>GMTTLNLNTLSERIKAHKMALVHIVKPPVCTERAQHYTEMYQQHMDKPIPVRRALALAHHLAQRTIWIKHDELIVGNQASEVRAAPIFPEYTVSWIEKEIDDLADRPGAGFAVSEENKRVLHEICPWWRGQTVQDRCYGMFTDEQKSLLETGIIKAEGNMTSGDAHLAVNFPLVLEKGLDGLRAKVAERRSRINLTVLDDLHGDQFLKAIDIVLEAVSLHIERFAALAREMAATESRVSRRDELLAIAENCDAIAHEPPKTFWQALQLCYFIQLILQIESNGHSVSFARMDQYLYPYYRRDVELNQSLDREHVIELLHSCWLKLLEVNKIRSGSHSKASAGSPLYQNVTIGGQKLVNGEPMDAVNPLSYAILESCGRLRSTQPNLSVRYHAGMSNDFLDACVQVIRCGFGMPAFNNDEIVIPEFIKLGVEKEDAYDYAAIGCIETAVGGKWGYRCTGMSFINFARVMLAALEGGRDATSGKVFLPQEKALSAGNFGNFDEVMTAWDTQIRYYTRKSIEIEYVVDTMLEENVHDILCSALVDDCIERAKSIKQGGAKYDWVSGLQVGIANLGNSLAAVKKLVFEQGVIGQQQLAAALADDFDGLTHEQLRQRLINGAPKYGNDDDSVDMLLTRAYQTYIDELKQYHNPRYGRGPIGGNYYAGTSSISANVPFGAATMATPDGRKAHTPLAEGASPASGTDHLGPTAVIGSVGKLPTEAILGGVLLNQKLNPSTLENDSDRQKLMVLLRTFFEVHKGWHIQYNI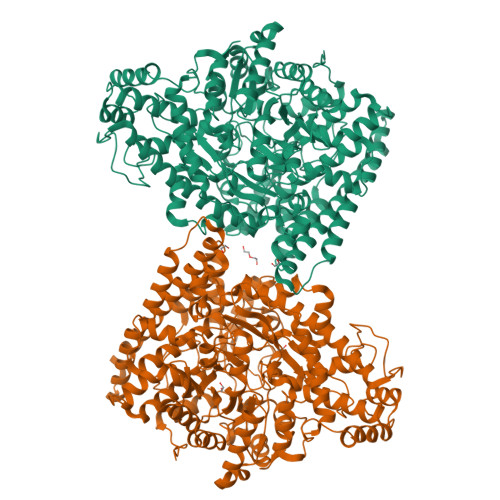VSRETLLDAKKHPDQYRDLVVRVAGYSAFFTALSPDAQDDIIARTEHTL[2x]>NVGKKYFMSSVRRMPLNRAKALCSELQGTVATPRNAEENRAIQNVAKDVAFLGITDQRTENVFEDLTGNRVRYTNWNEGE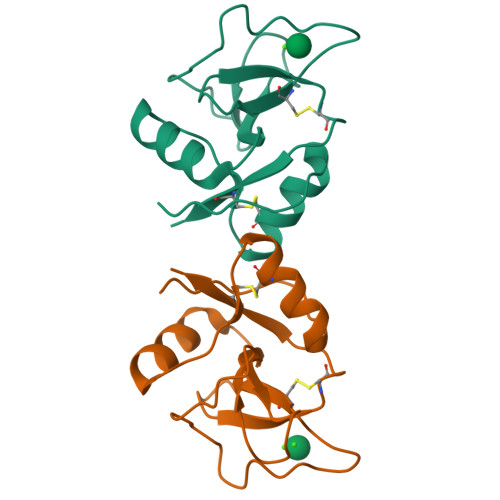PNNVGSGENCVVLLTNGKWNDVPCSDSFLVVCEFS[2x]> GSNAGGSSPITGLVYDQRMMLHHNMWDSHHPELPQRISRIFSRHEELRLLSRCHRIPARLATEEELALCHSSKHISIIKSSEHMKPRDLNRLGDEYNSIFISNESYTCALLAAGSCFNSAQAILTGQVRNAVAIVRPPGHHAEKDTACGFCFFNTAALTARYAQSITRESLRVLIVDWDVHHGNGTQHIFEEDDSVLYISLHRYEDGAFFPN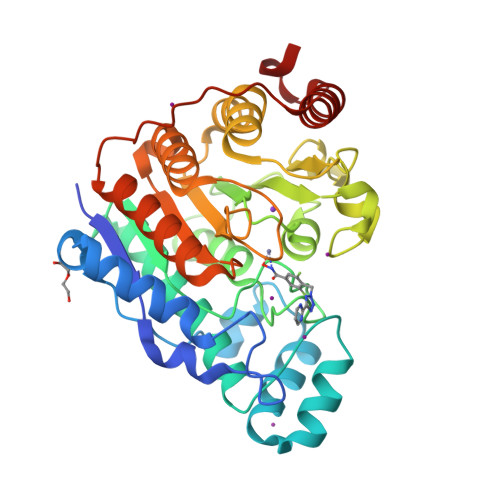SEDANYDKVGLGKGRGYNVNIPWNGGKMGDPEYMAAFHHLVMPIAREFAPELVLVSAGFDAARGDPLGGFQVTPEGYAHLTHQLMSLAAGRVLIILEGGYNLTSISESMSMCTSMLLGDSPPSLDHLTPLKTSATVSINNVLRAHAPFWSSLR>GMREDMKDNVVKDKSLEFAVRIVNLYKFLVNEQKEFVMSKQILRSGTSIGANIREAEQAQSRADFINKLNIAL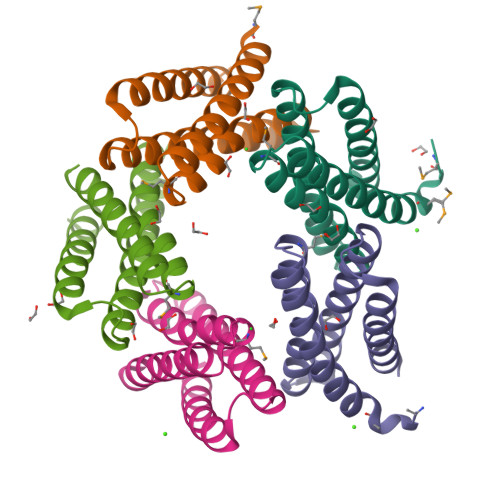KEANETEYWLELLIRTEYITREQYESINNDSTEINKLLISIIKTTKNN[5x]>[2x]SNAMIIADNIKQFHSIRNSLIKQQKIGFVPTMGALHNGHIS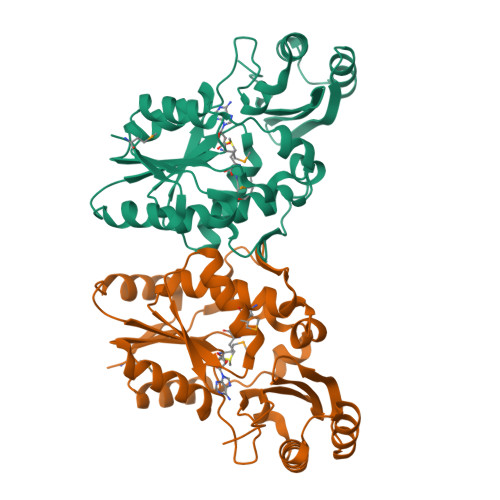LIKKAKSENDVVIVSIFVNPTQFNNPNDYQTYPNQLQQDIQILASLDVDVLFNPSEKDIYPDGNLLRIEPKLEIANILEGKSRPGHFSGMLTVVLKLLQITKPNNLYLGEKDYQQVMLIKQLVKDFFINTKIIVCPTQRQPSGLPLSSRNKNLTSTDIEIANKIYEILRQDDFSNLEELTNKINSTGAKLQYIQKLNNRIFLAFYIGKVRLIDNFLKETGPSC>[17x]MKKITLLLAGSALLLSGCAGVKSSFDCDATTSDTCMTMTKANQLARDKAAKQAGKPAAGGLPSLVNLPATSAVEVPSASRSAVTPPSGTRTVSTTPPVSAGTSAGVNTNTTTSTLTPRPVAGTPVTTTPSSVAYRPVVSVVTPTPSCQNVRCDNPGTVHPQRSRDQIATVWIAPWVDSDNAFHQPGRVSFVVSPADWVLPARVN;>[17x]MANVNKVVRRRQVALLIALVLGIGAGGAGTWMVSEMNLKKAPPAKAPKGEPAPDMTGVVNQSFDNKVQRSAIAEAQRLNKETQTEIKKLRTEMGLVSRDLKGSQDRIRELEDQNQLLQTQLEAGKNFDSLSAEPLPGALA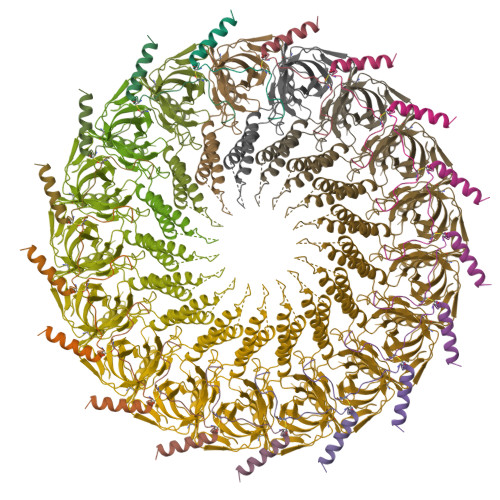SQGKPAPAGNVPPPTSFWPAGGGQAPAAPVMTPIQRPGMMDSQEFSLPDTGPKKPRFPWISSGSFVEAIVVEGADANASVTGDKNTAPMQLRLTGKVQMPNDEEFDLTGCFVTLEAWGDVSSERAIVRSRSISCKLGDDDIDQKIAGHVSFMGKNGIKGEVVMRNGQILLYAGGAGFLDGIGKGIEKASSTTVGVGATASMSAADIGQAGLGGGVSSAAKTLSDYYIKRAEQYHPVIPIGAGNEVTLVFQDGFQLETLEEARAKAAARKKQNQPSASSTPAAMPGNTPDMLKQLQDFRVGDTVDPATGQVVTQ>DPFAGDPPRHPGLRVNSQKPFNAEP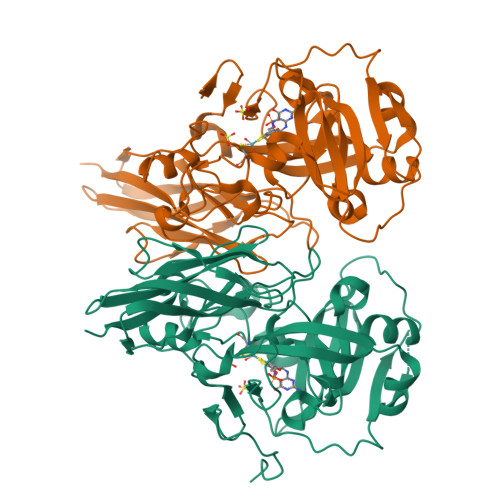PAELLAERFLTPNELFFTRNHLPVPAVEPSSYRLRVDGPGGRTLSLSLAELRSRFPKHEVTATLQCAGNRRSEMSRVRPVKGLPWDIGAISTARWGGARLRDVLLHAGFPEELQGEWHVCFEGLDADPGGAPYGASIPYGRALSPAADVLLAYEMNGTELPRDHGFPVRVVVPGVVGARSVKWLRRVAVSPDESPSHWQQNDYKGFSPCVDWDTVDYRTAPAIQELPVQSAVTQPRPGAAVPPGELTVKGYAWSGGGREVVRVDVSLDGGRTWKVARLMGDKAPPGRAWAWALWELTVPVEAGTELEIVCKAVDSSYNVQPDSVAPIWNLRGVLSTAWHRVRVSVQD[2x]> SGYSMTPPTLNITEESHVIDTGDSLSISCRGQHPLEWAWPGAQEAPATGDKDSEDTGVVRDCEGTDARPYCKVLLLHEVHANDTGSYVCYYKYIKARIEGTTAASSYVFVRDFEQPFINKPDTLLVNRKDAMWVPCLVSIPGLNVTLRSQSSVLWPDGQEVVWDDRRGMLVSTPLLHDALYLQCETTWGDQDFLSNPFLVHITG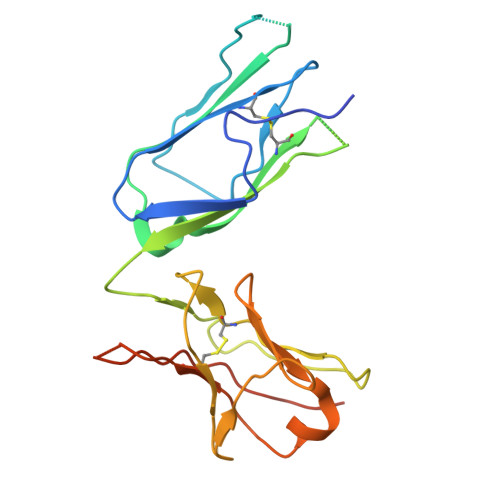NELADPIEGR>[2x]MHHHHHHASGLVP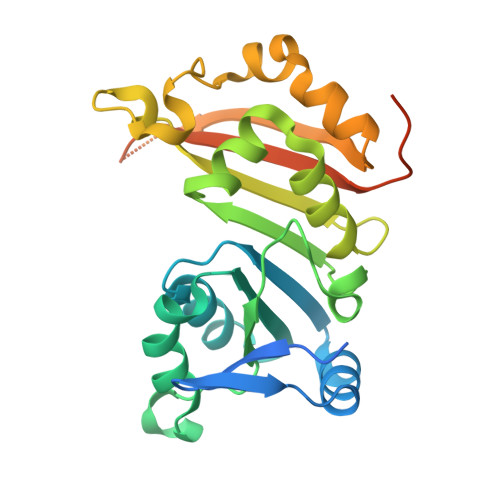RGSHMTRTTALKVLAGKKLTDLDPDEWAKAQASAERILVDVGTGDARTAYRQAIAHPEWLVVGVDPAWQRMTETAVRAARKPAKGGAPNLVLVSSAIETVPAALHGVADEVMVLMPWGKLLRGVVLGEADVLSGLRAVAKPGAPLEISIGTSIWREPIPLEIRDLPELTPETVVSTGLTDRLAALGWQVADVRLVPHTDLDTISSSAARRLGSGATETVLHLRAVAVDPRDPVGTQHPAAESAQDTPEEPQRDV> MDQECIENYAKVNGIYIYYKLCKAPEEKAKLMTMHGAPGMSHDYLLSLRDMTKEGITVLFYDQFGCGRSEEPDQSKFTIDYGVEEAEALRSKLFGNEKVFLMGSSYGGALALAYAVKYQDHLKGLIVSGGLSSVPLTVKEMNRLIDELPAKYRDAIKKYGSSGSYENPEYQEAVNYFY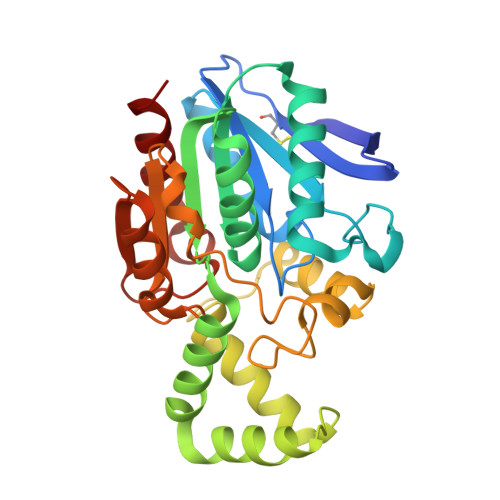HQHLLRSEDWPPEVLKSLEYAERRNVYRIMNGPNEFTITGTIKDWDITDKISAIKIPTLITVGEYDEVTPNVARVIHEKIAGSELHVFRDCSHLTMWEDREGYNKLLSDFILKHL> MSKYSQDVLQLLYKNKPNYISGQSIAESLNI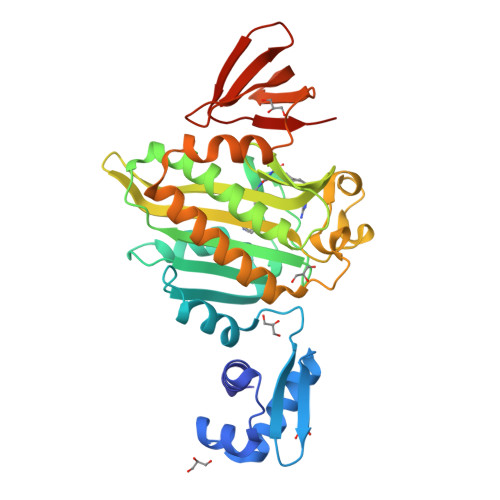SRTAVKKVIDQLKLEGCKIDSVNHKGHLLQQLPDIWYQGIIDQYTKSSALFDFSEVYDSIDSTQLAAKKSLVGNQSSFFILSDEQTKGRGRFNRHWSSSKGQGLWMSVVLRPNVAFSMISKFNLFIALGIRDAIQHFSQDEVKVKWPNDIYIDNGKVCGFLTEMVANNDGIEAIICGIGINLTQQLENFDESIRHRATSIQLHDKNKLDRYQFLERLLQEIEKRYNQFLTLPFSEIREEYIAASNIWNRTLLFTENDKQFKGQAIDLDYDGYLIVRDEAGESHRLISADIDFGHHHHHH> MGSSHHHHHHSQDPNSMTTLTRQDLNFGQVVADVLCEFLEVAVHLILYVREVYPVGIFQKRKKYNVPVQMSCHPELNQYIQDTLHCVKPLLEKNDVEKVVVVILDKEHRPVEKFVFEITQPPLLSISSDSLLSHVEQLLAAFILKISVCDAVLDHNPPGCTFTVLVHTREAATRNMEKIQ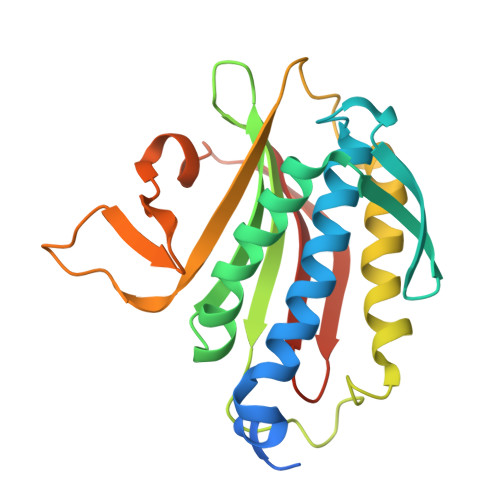VIKDFPWILADEQDVHMHDPRLIPLKTMTSDILKMQLYVEERAHKGS>MMYKEPFGVKVDFETGIIEGAKKSVRRLSDMEGYFVDERAWKELVEKEDPVVYEVYAVEQEEKEGDLNFATTVLYPGKVGKEFFFTKGHFHAKLDRAEVYVALKGKGGMLLQTPEGDAKWISMEPGTVVYVPPYWAHRTVNIGDEPFIFLAIYPADAGHDYG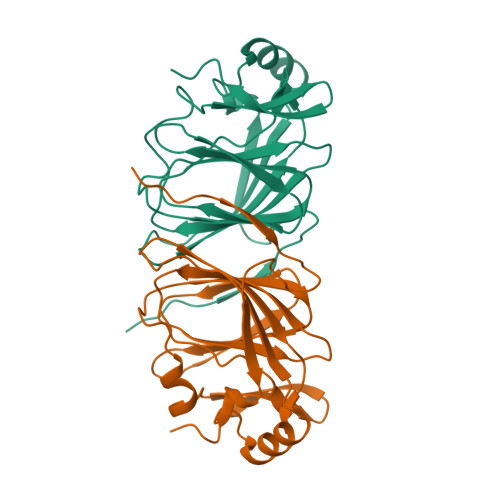TIAEKGFSKIVIEENGEVKVVDNPRWKK[2x]> MATKGTKRSYEQMETDGERQNATEIRASVGKMIDGIGRFYIQMCTELKLSDYEGRLIQNSLTIERMVLSAFDERRNKYLEEHPSAGKDPKKTGGPIYRRVDGKWRRELILYDKEEIRRIWRQANNGDDATAGLTHMMIWHSNLNDATYQRTRALVRTGMDPRMCSLMQGSTLPRRSGAAGAAVKGVGTMVMELIRMIKRGINDRNFWRGENGRRTRIAYERMCNILKGKFQTAAQRTMVDQVRESRNPGNAEFEDLIFLARSALILRGSVAHKSCLPACVYGSAVASGYDFEREGYSLVGIDPFRLLQNSQVYSLIRPNENPAHKSQLVWMACHSAAFEDLRVSSFIRGTKVVPRGKLSTRGVQIASNENMETMESSTLELRSRYWAIRTRSGGNTNQQRASSGQISIQPTFSVQRNLPFDRPTIMAAFTGNTEGRTSDMRTEIIRLMESARPEDVSFQGRGVFELSDEKATSPIVPSFDMSNEGSYFFGDNAEEYDNLEHHHHHH

Influenza virus genome encapsidation is essential for the formation of a helical viral ribonucleoprotein (vRNP) complex composed of nucleoproteins (NP), the trimeric polymerase, and the viral genome. Within each vRNP, the viral RNA (vRNA) segment is encapsidated by the viral nucleoprotein (NP) and attached to the heterotrimeric RNA-dependent RNA polymerase. In this study, we established a biological tool, the RNP-like particles assembled from recombinant influenza A virus NP and synthetic RNA, and we present the first subnanometric cryo–electron microscopy structure of the helical NP-RNA complex (8.7 to 5.3 Å). The RNP-like particles are a tool that mimics the influenza nucleocapsid.

The helical RNP-like structure reveals a parallel double-stranded conformation, allowing the visualization of NP-NP and NP-RNA interactions. Each asymmetric unit (NP monomer) is related by a rise of 24.3 Å and a twist of 57.4°, resulting in a right-handed parallel double-stranded helical reconstruction with approximately 6.3-NP protomers per helix turn. Close examination of Laplacian-filtered AFM images revealed grooves pointing toward the upper-right in regard to the central axis of the helix, which is characteristic of a right-handed helix conformation. Combined with the AFM data, these results confirm that our RNP-like particles are assembled as a right-handed helix. We were able to visualize a parallel double-stranded helical assembly at a resolution sufficiently high to describe the conformational changes of NP to accommodate RNA binding and oligomerization into nucleocapsid. It is important to point out that our helical reconstruction is straight and does not fully reflect the highly flexible nature and the inherent dynamic of our ribonucleoprotein-like particles and so the vRNP. Like every model, there are limitations; for one, the reconstituted RNPs form a double parallel helix as opposed to the antiparallel helix of native vRNP, most likely due to the short RNA and the absence of the polymerase. The RNP-like structure resembles the compacted state of vRNP; however, because of the parallel helical assembly, this structure can only provide meaningful information regarding the intra-strand interactions such as the NP-NP oligomerization, NP-RNA interaction, and overall architecture along one strand. We did not observe interstrand interactions that would be relevant for vRNP coherence. To propose a picture even closer to that of a vRNP, we generated the antiparallel RNP-like conformation by flipping one strand by 180° around an axis perpendicular to the helical axis without any steric clashes.Here, we have used metagenome-based technologies to identify and characterize novel bacterial lipolytic enzymes which catalyze both hydrolysis and esterification reactions at temperatures above 70°C. Metagenomic libraries from enriched soil and water samples were constructed and screening revealed two novel lipases designated LipS and LipT which showed a high temperature optimum and also a high stability against thermal denaturation. LipS assumes the fold of a classical α/β hydrolase. The active site of LipS is formed by the catalytic triad S126, D227 and H257 with the catalytic serine located at the sharp γ-turn between β4 and αD. The position of the catalytic triad and the oxyanion hole (F58 and M127) at conserved topological sites clearly designates this newly characterized enzyme as a hydrolase.

The initial construct LipS-H6 in SG P42212 diffracted X-ray radiation to 2.80 Å resolution, while a second construct, LipS-WT, diffracted X-ray radiation to 1.99 Å resolution. After refinement, the active site of LipS-WT in SG P4 contained strong residual density immediately adjacent to S126 and H257. This density was interpreted with spermidine. Spermidine was used as an additive to improve crystal quality and was subsequently shown to inhibit the activity of LipS with its substrate pNP-decanoate in concentration dependent manner. The terminal amino-group of spermidine comes remarkably close to both S126 and H257 when the secondary amid group interacts with D187, which lines the end of the active site cavity. Thus, it is likely that spermidine mimics substrate bound in the active site. At this point, there is no indication that spermidine is part of any native substrate of LipS. The conformations of the inserted domains in all four LipS molecules found in one asymmetric unit were identical. Furthermore, data that the inserted domain assumes the same conformation with and without bound spermidine in structures of LipS suggests that this is rather a rigid structure. Identical conformations of the lid-domain, which covers the active site, in the absence and presence of a ligand, indicate that this domain may not undergo conformational rearrangements during the catalytic cycle.

>[4x]GAMCRKSRNCRNPPRSGDAQQRPRERSGSGMSTTPLQVLPGAEPLYSVGSRIGVLVSHGFTGSPQSMRFLAEGFARAGYTVATPRLTGHGTTPAEMAASTASDWTADIVAAMRWLEERCDVLFMTGLSMGGALTVWAAGQFPERFAGIMPINAALRMESPDLAALAFNPDAPAELPGIGSDIKAEGVKELAYPVTPVPAIKHLITIGAVAEMLLPRVKCPALIIQSREDHVVPPHNGELIYNGIGSTEKELLWLENSYHVATLDNDKELILERSLAFIRKH>[2x]DPFTQFKQTPLPYAYDALEGAIDAKTMEIHHSKHAAGYTANLNKAIAGTPAEKESIENILAKVSQYSDAVRNNAGGHYNHELFWSILTPNKGTKPSAALQKAIDETFGSLDALKEKINAAGA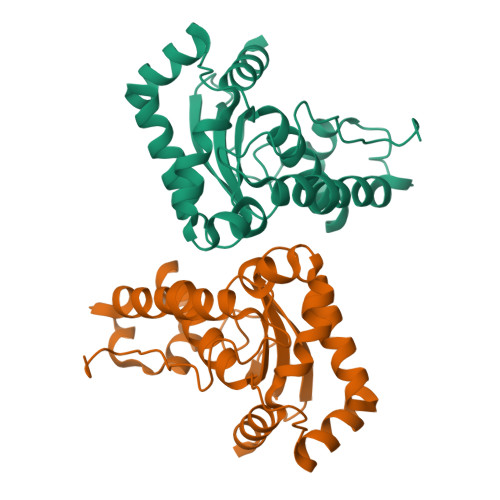ARFGSGWAWLIVDNGGKLQVTSTPNQDNPLMDFTKEKGTPILGIDVWEHAYYLRYQNKRADYLTTIWDVINWEEVSARYEKALK>[14x]MEQAMRERSELARKGIARAKSVVALAYAGGVLFVAENPSRSLQKISE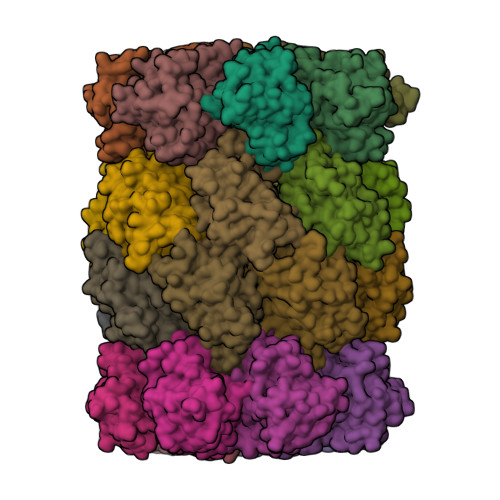LYDRVGFAAAGKFNEFDNLRRGGIQFADTRGYAYDRRDVTGRQLANVYAQTLGTIFTEQAKPYEVELCVAEVAHYGETKRPELYRITYDGSIADEPHFVVMGGTTEPIANALKESYAENASLTDALRIAVAALRAGSADTSGGDQPTLGVASLEVAVLDANRPRRAFRRITGSALQALLVDQESPQSDGESSG;>[14x]TTIVALKYPGGVVMAGDRRSTQGNMISGRDVRKVYITDDYTATGIAGTAAVAVEFARLYAVELEHYEKLEGVPLTFAGKINRLAIMVRGNLAAAMQGLLALPLLAGYDIHASDPQSAGRIVSFDAAGGWNIEEEGYQAVGSGSLFAKSSMKKLYSQVTDGDSGLRVAVEALYDAADDDSATGGPDLVRGIFPTAVIIDADGAVDVPESRIAELARAIIESRSGADTFGSDGGEKHHHHHH The canonical NuA3 complex acetylates histone H3, generating primarily the epigenetic mark H3K14ac3, and consists of five core subunits: the catalytic subunit Sas3 (something about silencing 3) and the nonenzymatic subunits Nto1 (NuA three ORF1), Eaf6 (Esa1p associated factor 6), Yng1 (yeast inhibitor of growth protein 1) and Taf14 (transcription initiation factor subunit 14). Taf14 is a core component of several chromatin associating complexes that regulate gene expression, DNA damage response and cytoskeletal organization in yeast cells. Here, we report that the Taf14 subunit of the NuA3 complex binds to two other subunits of the complex, Yng1 and Sas3, and describe the molecular mechanism by which the extra-terminal domain of Taf14 recognizes the conserved motif present in Yng1 and Sas3. The plant homeodomain (PHD) finger of Yng1 binds to (or reads) trimethylated lysine 4 of H3 (H3K4me3), whereas the YEATS (Yaf9, ENL, AF9, Taf14, Sas5) domain of Taf14 recognizes acylated lysine 9 of H3 (H3K9acyl)11–14.

To gain insight into the binding mechanism, we co-crystallized Taf14ET and Yng1EBM and determined the structure of the Taf14ET-Yng1EBM complex refining it to a 1.9 Å resolution. In the crystal structure, Taf14ET forms a head-to-toe dimer, which creates a deep, elongated binding groove for dimeric Yng1EBM, and mass photometry data indicate that the Taf14FL-Yng1EBM complex can also form a dimer in solution. Each Taf14ET monomer, colored light blue and wheat, folds into a three-helix bundle and a two-stranded anti-parallel β-sheet linking helices α2 and α3. The α1 helices of both Taf14ET monomers (α1 and α1’) are packed against each other in an antiparallel manner. The α1-α1’ dimerization interface of Taf14ET is stabilized through van der Waals and hydrophobic contacts. Dimeric Yng1EBM forms a long two-stranded anti-parallel β-sheet (one β strand is colored yellow, and another is red), which pairs with the β2 and β2’ strands from Taf14ET monomers and is restrained through extensive intermolecular interactions. Symmetric β-sheet contacts are observed between the backbone amides of L122, I120 and L118 of each Yng1EBM strand and G218, F220 and I222 of the respective β2 and β2’ strands of Taf14ET. The side chain amino groups of K115, K119 and K124 of Yng1EBM form salt bridges with the carboxyl groups of D223, E219 and E191 of Taf14ET, and the side chain amino group of K123 of Yng1EBM shares a hydrogen bond with the backbone carbonyl group of E216 of Taf14ET. The Yng1EBM-binding groove of the Taf14ET dimer is large and hydrophobic, and two molecules of Taf14ET almost encircle the dimeric Yng1EBM. The side chains of L117, L118, I120 and L122 from both strands of Yng1EBM are oriented toward and essentially buried in the hydrophobic groove.

>[4x]SVKGSVDLEKLAFGLTKLNEDDLVGVVQMVTDNKTPEMNVTNNVEEGEFIIDLYSLPEGLLKSLWDYVKKNT;>EPKLLLKINLKK[4x]Fibrillarin (FBL) is an essential and evolutionarily highly conserved S-adenosyl methionine (SAM) dependent methyltransferase. It is the catalytic component of a multiprotein complex that facilitates 2′-O-methylation of ribosomal RNAs (rRNAs), a modification essential for accurate and efficient protein synthesis in eukaryotic cells. Fibrillarin consists of an N-terminal glycine–arginine-rich domain (GAR), which is believed to be important for organisation of the nucleolus, and a C-terminal domain with a Rossmann fold that is characteristic of class I S-adenosylmethionine (SAM)-dependent methyltransferases. In the present study, we determined, to our knowledge, the first crystal structures of hFBL in ligand-free state, bound to the native cofactor SAM, and in complex with two fragments that can compete with SAM for binding to the cofactor site.

Fragment screening was carried out via both 19F NMR spectroscopy and X-ray crystallography using a library of 388 fluorinated compounds with great structural diversity. This library was originally assembled for 19F NMR detected screening, with the compounds grouped into 20 pools, each of which consists of up to 20 compounds. However, the robust crystallisation system we established for hFBL allowed us to apply exactly the same set of pools for crystallographic screening, and bound fragments were unambiguously identified from the electron density map. Compound 1 binds to the adenosine region of the hFBL cofactor binding site by an induced fit mechanism, which involves a significant rearrangement in the loop connecting the β4 strand and α5 helix. The compound induces a significant shift of the protein backbone around D236-Q242 resulting in extensive movement of the side chains of V237 (5.9 Å) and Q242 (5.2 Å). The movement of the side chain of V237, which forms a hydrophobic interaction with the adenine moiety of SAM in hFBLSAM, results in displacement of the side chain of Q242 from a buried to a solvent exposed position, and exposure of a new hydrophobic pocket (L166, A235, V237, I245, and V246) that accommodates the trifluoromethyl group of the compound. Compound 1 also forms hydrogen bonds with the side chain carboxylate of E191, the backbone nitrogen of F192, and a water molecule that interacts with the backbone nitrogen of A217 and the backbone carbonyl of E216. One of these fragment complexes (compound 1) revealed structural plasticity at the cofactor site as binding of the fragment lead to exposure of a hydrophobic cavity that accommodated the tri-fluoro moiety of the compound. Our discovery of conformational dynamics and a hydrophobic cavity at the hFBL cofactor site will help to facilitate structure-guided design of hFBL inhibitors.

>[2x]SNAGKNVMVEPHRHEGVFICRGKEDALVTKNLVPGESVYGEKRVSISEGDDKIEYRAWNPFRSKLAAAILGGVDQIHIKPGAKVLYLGAASGTTVSHVSDIVGPDGLVYAVEFSHRSGRDLINLAKKRTNIIPVIEDARHPHKYRMLIAMVDVIFADVAQPDQTRIVALNAHTFLRNGGHFVISIKANCIDSTASAEAVFASEVKKMQQENMKPQEQLTLEPYERDHAVVVGVYRPPPKVKN> DTHWFHRNPLKATAPVSFNYYGVVTGPSASKICNDLRSSRARLLELFTDLSCNPEMMKNAADSYFSLLQGFINSLDESTQESKLRYIQNFKWTDTLQGQVPSAQQDAVFELISMGFNVALWYTKYASRLAGKENITEDEAKEVHRSLKIAAGIFKHLKESHLPKLITPAEKGRDLESRLIEAYVIQCQAEAQEVTIARAIELKHAPGLIAALAYETANFYQKADHTLSSLEPAYSAKWRKYLHLKMCFYTAYAYCYHGETLLASDKCGEAIRSLQEAEKLYAKAEALCKEYGETKGPGPTVKPSGHLFFRKLGNLVKNTLEKCQRENGFIYFQKIPTEAPQLELKANYGLVEPIPFEFP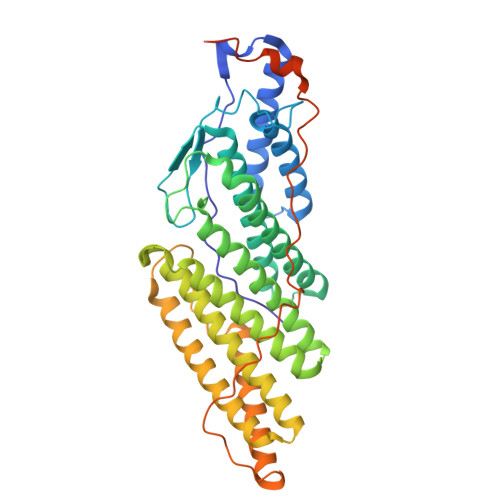PTSVQWTPETLAAFDLTKRPKDDSTKPKPEEEVKPVKEPDIKPQKDTGCYIS> MKVDGIQAEMRAMMVEATNTAPTASGAKVG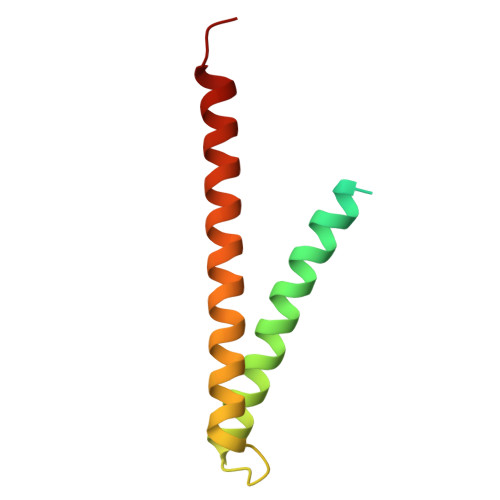ADFNDLLTKAINNVNTLQKASGDLQTRFDRGDADVSLSDVMIARNKSSVAFDATVQIRNKLVEAYKDLMNMPV>QDLMASGNTTVKATFGKDSSVVKWVVL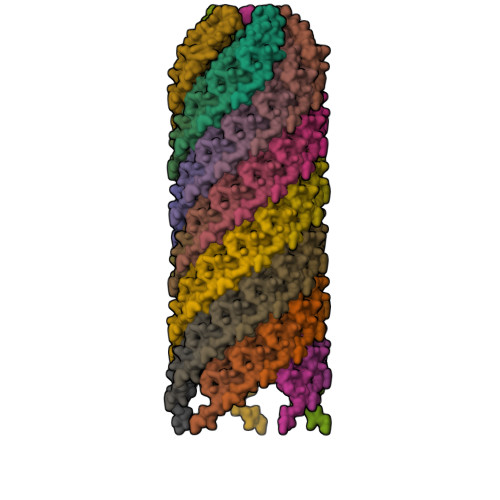AEVLVGAVMYMMTKNVKFLAGFAIISVFIAVGMAVVGL[75x]> XFAAAVGLAAPQVPA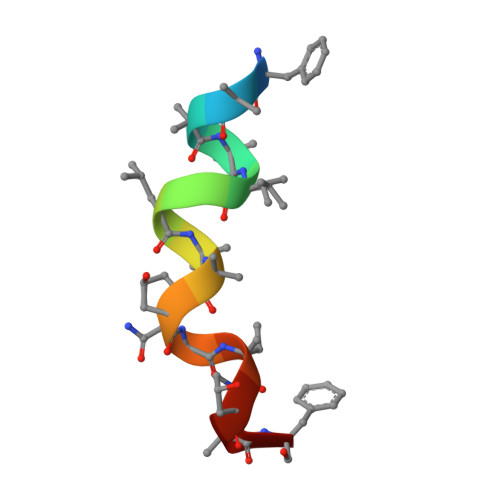F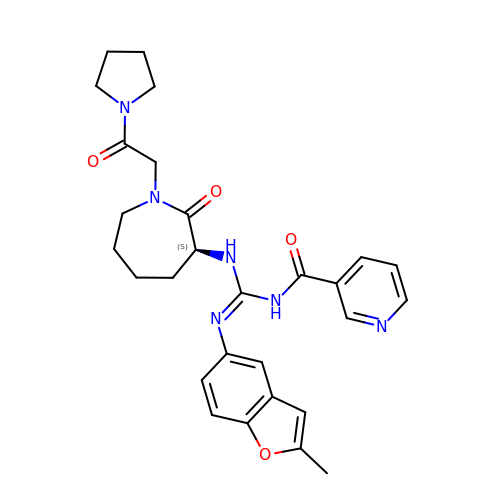N-{N'-(2-methyl-1-benzofuran-5-yl)-N-[(3S)-2-oxo-1-(2-oxo-2-pyrrolidin-1-ylethyl)azepan-3-yl]carbamimidoyl}pyridine-3-carboxamide | C28 H32 N6 O4 | GNYXHJVKEWBHAI-QHCPKHFHSA-N> SVATV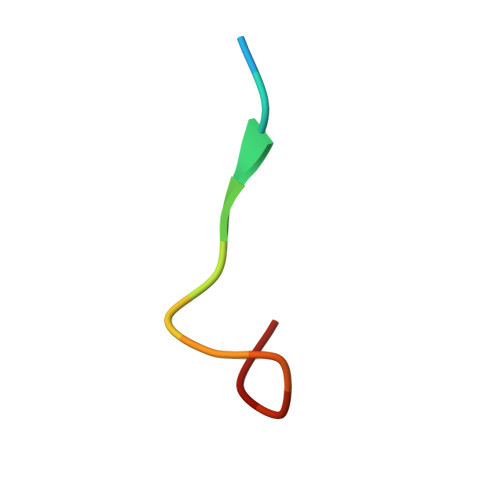SESLLTE>MKEVTIEIKNKTGLHARPAALFVQTASKFSSQIWVEKDNKKVNAKSIMGIMSLGVSQGNVVKLSA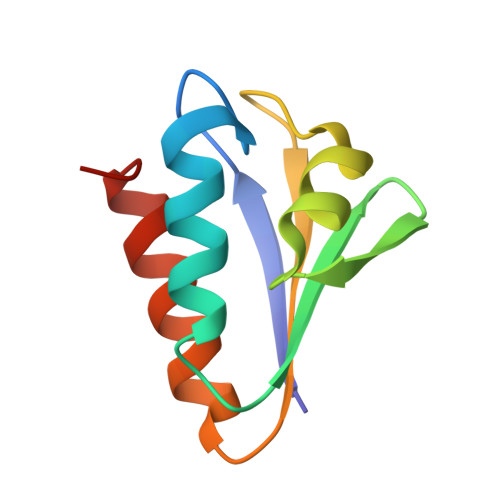EGDDEEEAIKALVDLIESKFGEE[3x]> VLRSKSLCHDEIENLLDSDHRELIGDYSKAFLLQTVDGKHQDLKYISPETMVALLTGKFSNIVDKFVIVDCRYPYEYEGGHIKTAVNLPLERDAESFLLKSPIAPCSLDKRVILIFHCEFSSERGPRMCRFIRERDRAVNDYPSLYYPEMYILKGGYKEFFPQHPNFCEPQDYRPMNH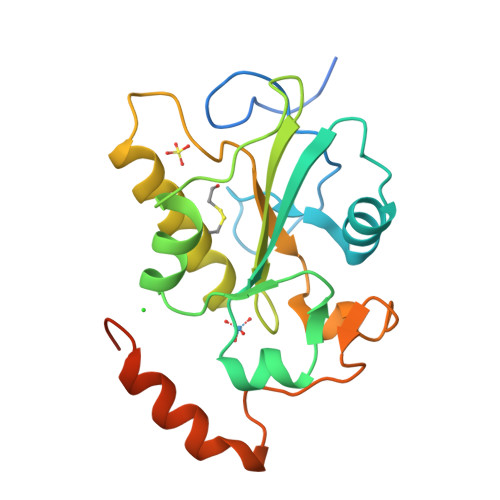EAFKDELKTFRLKTRSWAGERSRRELCSRLQDQ>SQVSTEFIPTRIAILTVSNRRGEE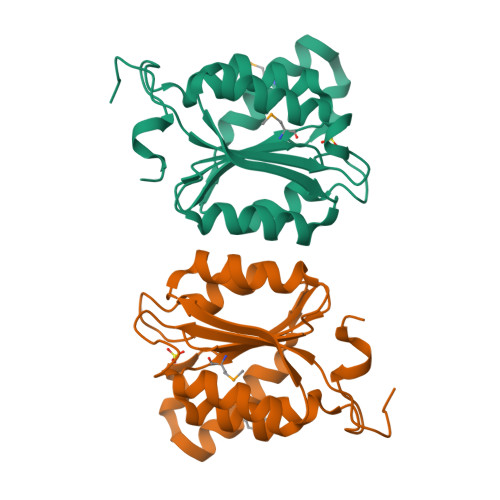DDTSGHYLRDSAQEAGHHVVDKAIVKENRYAIRAQVSAWIASDDVQVVLITGGTGLTEGDQAPEALLPLFDREVEGFGEVFRMLSFEEIGTSTLQSRAVAGVANKTLIFAMPGSTKACRTAWENIIAPQLDARTRPCNFHPHLKK[2x]>MELKHSISDYTEAEFLQLVTTICNADTSSEEELVKLVTHFEEMTEHPSGSALIYYPKEGDDDSPSGIVNTVKQWRAANGKSGFKQG[2x];>MESKRNKPGKATGKGKPVGDKWLDDAGKDSGAPIPDRIADKLRDKEFKSFDDFRKAVWEEVSKDPELSKNLNPSNKSSVSKGYSPFTPKNQQVGGRKVYELHHDKPISQGGEVYDMDNIRVTTPKR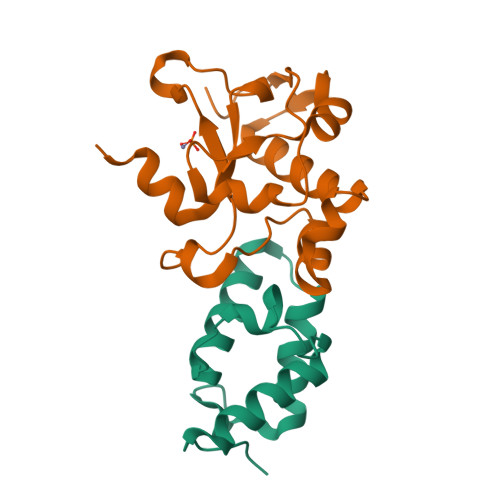HIDIHRGK[2x]>MGAMIVKEVYETAEKIKSMEIRGAGRIARAAAQALMIQAEKSKAKEPEELWNELKVASKILYNTRPTAVSLPNALRYVMHRVKAAYLGGADLETLRFTAINSAKEFIYNSEKAIERIGEIGAKRIEDGDIIMTHCHSKAAISVMKKAFEQGKNIKVIVTETRPKWQGKITAKELASYGIPVIYIVDSAARHYMKMTDKVVMGADSITANGAVINKIGTSLIALTAKEHRVWVMIAAETYKFHPATMLGQLVEIEMRDPTEVIPE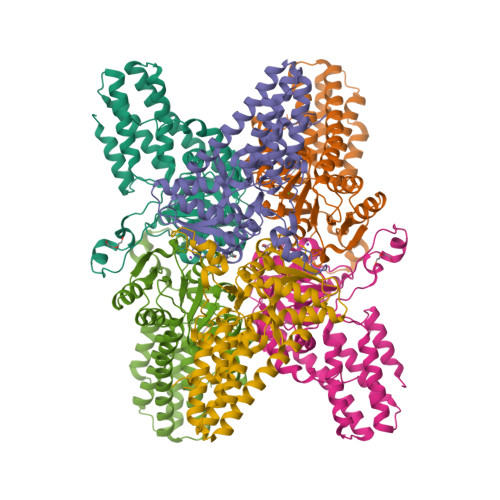EELRTWPKNIEVWNPAFDVTPPEYIDVIITERGIIPPYAAIDILKEEFGWALKYKEPWED[3x]> MPLLSASIVSAPVVTSETYVDIPGLYLDVAKAGIRDGKLQVILNVPTPYATGNNFPGIYFAIATNQGVVADGCFTYSSKVPESTGRMPFTLVATIDVGSGVTFVKGQWKSVR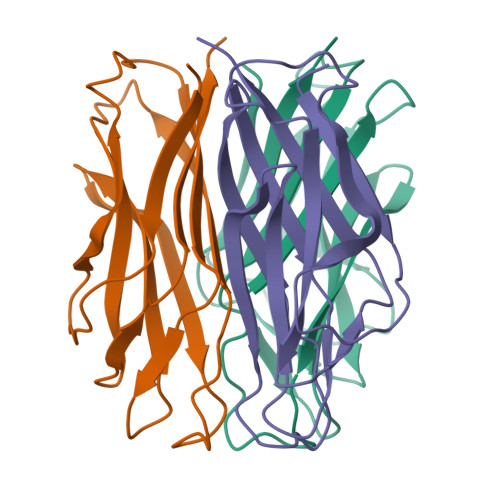GSAMHIDSYASLSAIWGTA> MVAVEQSEASRLGPVFDSCRANNRAALIGYLPTGYPDVPASVAAMTALVESGCDIIEVGVPYSDPVMDGPTIARATEAALRGGVRVRDTLAAVEAISIAGGRAVVMTYWNPVLRYGVDAFARDLAAAGGLGLITPDLIPDEAQQWLAASEEHRLDRIFLVAPSSTPERLAATVEASRGFVYAASTMGVTGA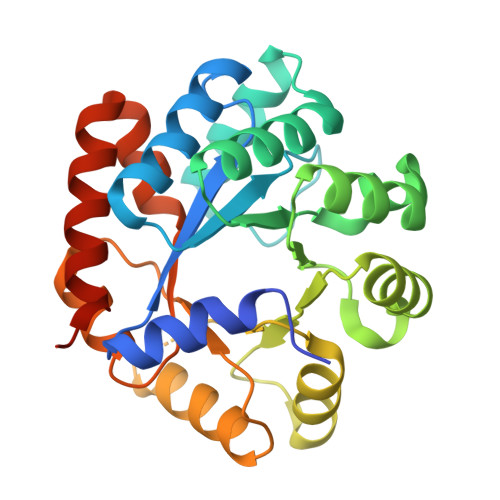RDAVSQAAPELVGRVKAVSDIPVGVGLGVRSRAQAAQIAQYADGVIVGSALVTALTEGLPRLRALTGELAAGVRLGMSAHHHHHH> VTVTVNKNPSHTVPSTLYGLMFEDINHSGDGGLYAELLQNRAFQQVTPNTAAALAAWHPISNAKLAVIQDPSPVSNALPNSLQFSVPSGSSGRVGFTNEGFWGIKVDSTWTYKASLFFRFPTSSSFSGALTVGLQTNAGRVLAQNSTQIRGTTTKWTQIN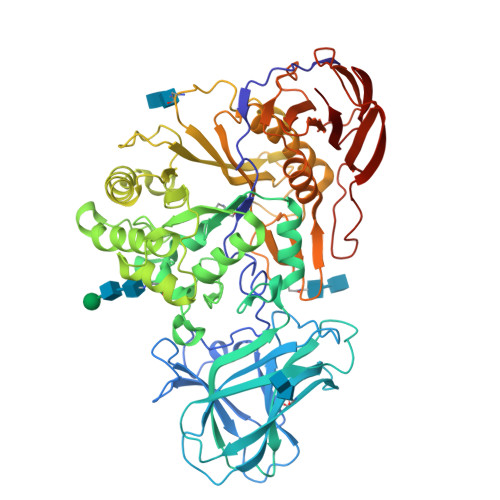LELHPTASAPDVSNSFFVTIDGAAGAGQTINFAMFSLFPPTFKNRPNGLRADIAETLAEMGPSFFRFPGGNNLEGQTTATRWQWNATVGSLLDRPGRVGDWGYVNTDGLGLLEYLQFFEDTGMEPIMAVWAGYSLGGTSLAENQLAPYIQQAIDQINFVIGDPAKSAPAALRASLGHPEPFTLRFVEVGNEDFFAAGSYPYRWHDFVTALQAQFPQIRFIATTNAWNPVLSPVPQSYDVHVYQTPTWFYQNAFYYDGFQRNGTTYFEGEYAAISTNANDLFGTVADGRLAFPTVQSATGEAAFMTGLERNSDIVFAASYAPLLQHVNSTQWTPDLVSYDAGSVIKSTSFFAQKLFALNKGDQYLPSTLPTNGGTLHWSITRASSSGKTFIKIANAGSSAQSLTFQLTQFNSVSSTGTLQVLTGPETASNTPEAPQAIVPKTSTIGTGKTFTYNAPAFSVSVITVTTN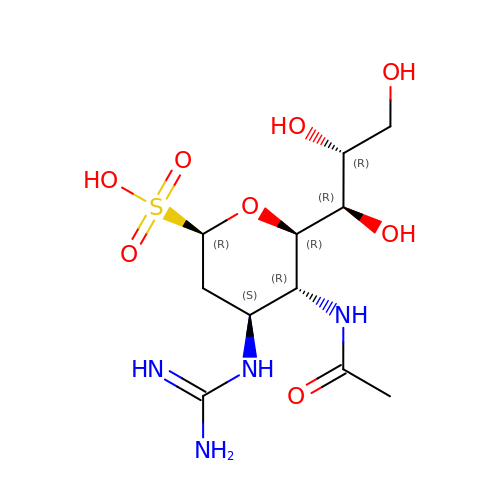(1R)-4-acetamido-1,5-anhydro-3-carbamimidamido-2,3,4-trideoxy-1-sulfo-D-glycero-D-galacto-octitol | C11 H22 N4 O8 S | SMAXKAOIZYKFEF-IHICSVBISA-N>[2x]GPVDMTERLKVMTIFGTRPEAIKMAPLVLELQKHPEKIESIVTVTAQHRQMLDQVLSIFGITPDFDLNIMKDRQTLIDITTRGLEGLDKVMKEAKPDIVLVHGDTTTTFIASLAAFYNQIPVGHVEAGLRTWDKYSPYPEEMNRQLTGVMADLHFSPTAKSATNLQKENKDESRIFITGNTAIDALKTTVKETYSHPVL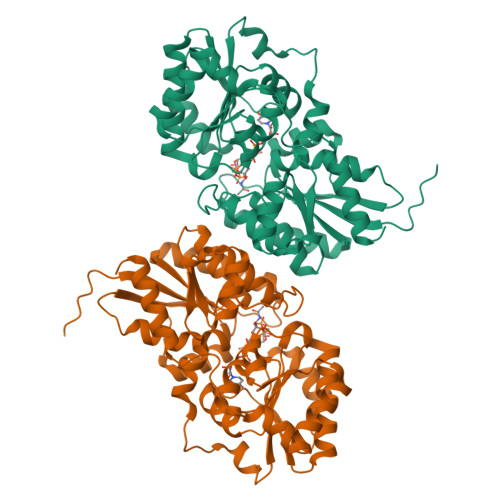EKLGNNRLVLMTAHRRENLGEPMRNMFRAIKRLVDKHEDVQVVYPVHMNPVVRETANDILGDYGRIHLIEPLDVIDFHNVAARSYLMLTDSGGVQEEAPSLGVPVLVLRDTTERPEGIEAGTLKLAGTDEETIFSLADELLSDKEAHDKMSKASNPYGDGRASERIVEAILKHFNK> 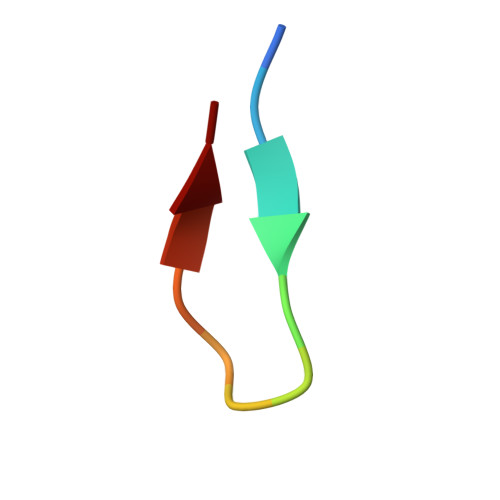SDKENFWGMAVA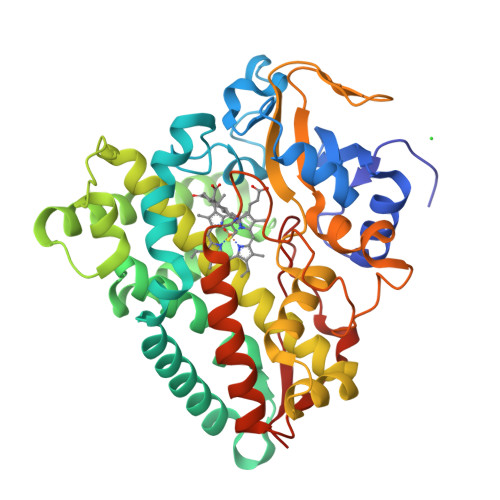>[2x]MNACPHSDTLTIDPMITDLAGETSRLRAAGPLTRIDLLGVPALAVTGHTLARQLLTDTRLVKDINAWSLWQSGTVTRQWPLIGMIDVDRSMFTVDGPEHRRLRIKTTQALTRRRLDALKPTIERYVAELLDDLERAGADGAVVDLKSVFAYPLPMRVISALMGVPSEDQEQLLTWYKAFFSILTPQDERLRVIDEMHGYFTEMVRRKTAEPGDDLTSALIYATDGETPLTEEEVIGNLQALVAAGHETTVSLILTAVRALLSHPEQLRLVRDGEIGWETAIEETLRWDGPVIHLLMRFATEDIDLGDAVIPRGEGVVMSYRAIGRDITVHGADADDFDITRATAARHISFGHGPHICPGAALARLEAAIALPALFTRFPHLHPALPLDQIPNLPVLTQNDLSHFPIHLG>KVFERCELARTLKRLGMDGYRGISLANWMCLAKWESGYN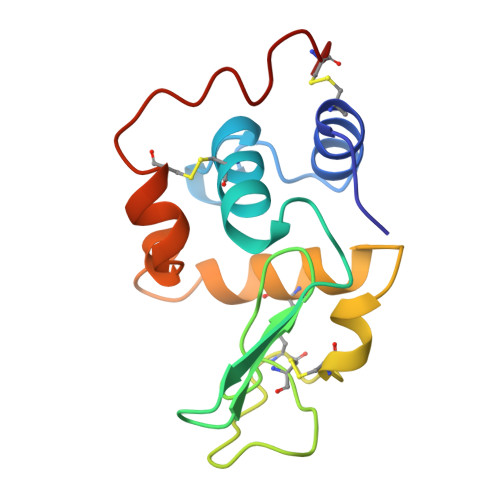TRATNYNAGDRSTDYGIFQINSRYWCNDGKTPGAVNACHLSCSALLQDNIADAVACLKRVVRDPQGIRAHVAWRNRCQNRDVRQYVQGCGV[2x]E)-10-[(3-Chloro-6,7,10,11-tetrahydro-9-methyl-7,11-methanocycloocta[b]quinolin-12-yl)amino]-N-(4-hydroxy-3-methoxybenzyl)-6-decenamide 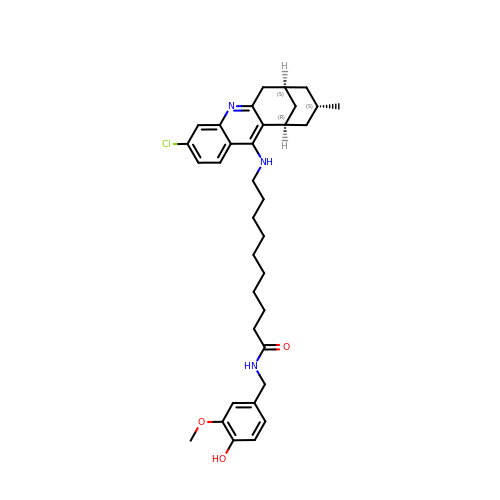| C35 H46 Cl N3 O3 | QVNUYAPHLZOXQT-AYRHNUGRSA-N>[2x]MKKGHHHHHHGEVSREKITLLRELGQGSFGMVYEGNARDIIKGEAETRVAVKTVNESASLRERIEFLNEASVMKGFTCHHVVRLLGVVSKGQPTLVVMELMAHGDLKSYLRSLRPEAENNPGRPPPTLQEMIQMAAEIADGMAYLNAKKFVHRDLAARNCMV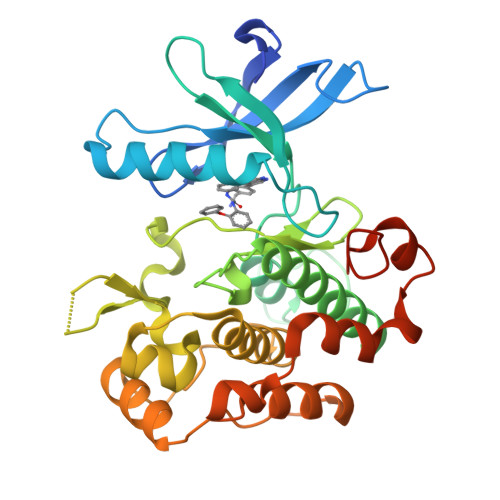AHDFTVKIGDFGMTRDIYETDYYRKGGKGLLPVRWMAPESLKDGVFTTSSDMWSFGVVLWEITSLAEQPYQGLSNEQVLKFVMDGGYLDQPDNCPERVTDLMRMCWQFNPKMRPTFLEIVNLLKDDLHPSFPEVSFFHSEENKAPESEELEMEFE>MKKYTCTVCGYIYNPEDGDPDNGVNPGTDFKDIPDDWVCPLC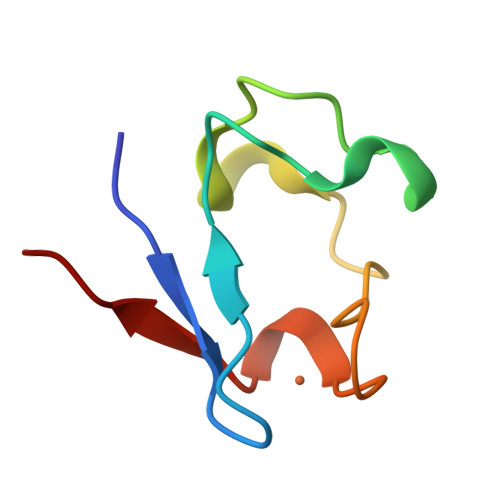GAPKDQFEEVEE[3x]>[2x]GPMSSVQLSRGDFHSIFTNKQRYDNPTGGVYQVYNTRKSDGANSNRKNLIMISDGIYHMKALLRNQAASKFQSMELQRGDIIRVIIAEPAIVRERKKYVLLVDDFELVQSRADMVNQTSTFLDNYFSEHPNETL;>[2x]GPMADLWDDNDDDDDILELVNRPPMSQMAVPIKPPESQAEQLMKAKGEVGVLRQKLSMLEKTLREHDDNQKKLESSLKS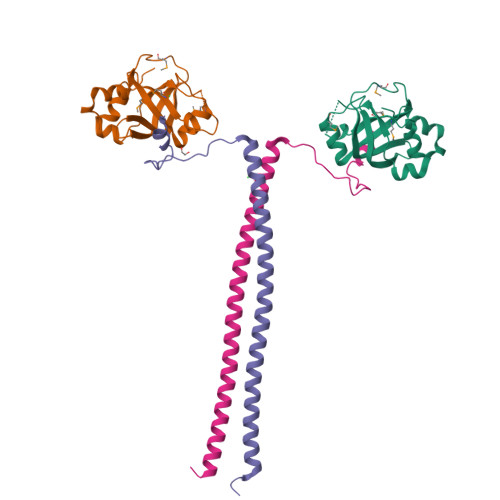SHEEEVTKLKIELERLEDERKFMLLEQKHLFT3-cyclopropyl-1-{5-methyl-2-[(3-methyl-1,2-thiazol-5-yl)amino]pyrimidin-4-yl}azetidin-3-ol 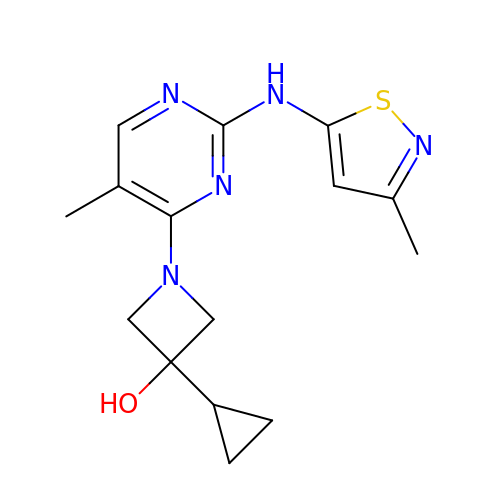| C15 H19 N5 O S | AYYRUOOCJNTWHJ-UHFFFAOYSA-N> VEKK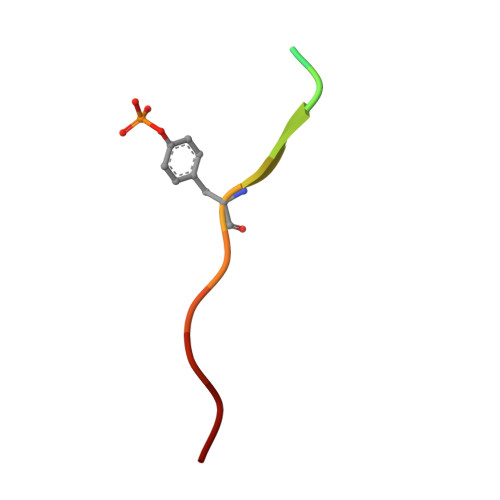SLTIYAQVQK> GRKEKVVLKIASIAPARSIWETELKKLSAEWSEITGGLVSMKFYDMSSLGGEREGIRKLKSSRPGQAAPLDGAVFSCLGLSELAPDSGIYTLSVPFLIQNEKDLERVLHELREDLDRPFRAAGFRVITWTNAGWLSFYTRAPYASLGQLKKQTIALSSLDSSVLGTCFRICGFDIKDAPNVRLAPLLKAGSIDGFLSVHLFTWATGFYRYISYALD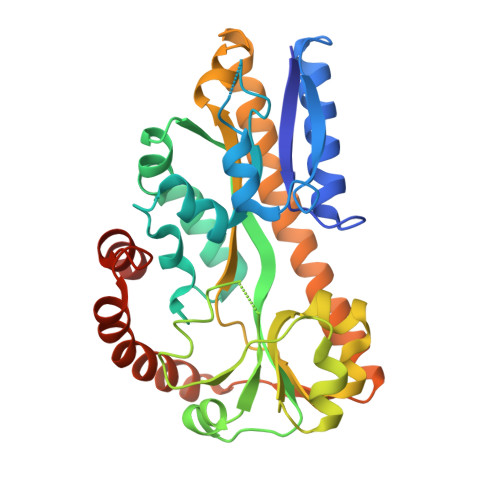TKICPAVIGMLISDGSWARIPSRYHDAMLQAATRVRQRLANNLETLDRECSNNIQKAGVSIVHLTPQEIQEWRTEFAADVKRIQARLPGMLNMTLYEKIKHLLYSAQR> LSLRQS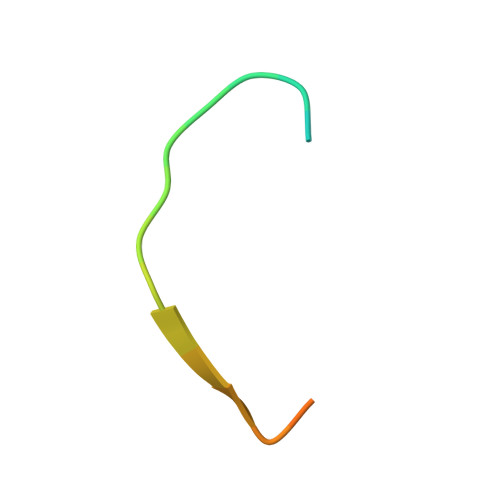IRFFKPATRTLCSSRYLL>MAHHHHHHMTELFIDGAWVDGAGPVFASRNPGTNERVWEGASASADDVERAVASARRAFAAWSALDLDARCTIVKRFAALLVERKEALATMIGRETGKPLWEARTEVASMAAKVDISITAYHERTGEKRAPMADGVAVLRHRPHGVVAVFGPYNFPGHLPNGHIVPALIAGNTVVFKPSELAPGVARATVEIWRDAGLPAGVLNLVQGEKDTGVALANHRQIDGLFFTGSSDTGTLLHKQFGGRPEIVLALEMGGNNPLVVAEVEDIDAAVHHAIQSAFLSAGQRCTCARRILVPRGAFGDRFVARLADVASKITASVFDADPQPFMGAVISARAASRLVAAQARLVGLGASPIIEMKQRDPALGFVNAAILDVTNVRELPDEEHFGPLAQIVRYTDLDDAIARANDTA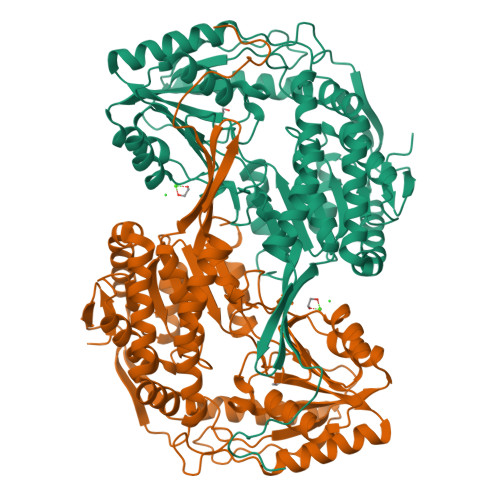FGLSAGLLADDEQAWHTFRRAIRAGIVNWNRPTNGASSAAPFGGAGRSGNHRPSAYYAADYCAYPMASVESAQLQMPASLSPGLHF[2x]> PITGLVYDQRMMLHHNMWDSHHPELPQRISRIFSRHEELRLLSRCHRIPARLATEEELALCHSSKHISIIKSSEHMKPRDLNRLGDEYNSIFISNESYTCALLAAGSCFNSAQAILTGQVRNAVAIVRPPGHHAEKDTACGFCFFNTAALTARYAQSITRESLRVLIVDWDVHHGNGTQHIFEEDDSVLYISLHRYEDGAFFPNSEDANYDKVGLGKGRGYNVNIPWNGGKMGDPEYMAAFHHLVMPIAREFAPELVLVSA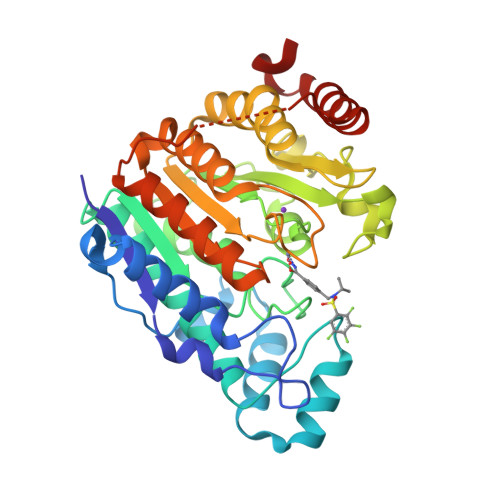GFDAARGDPLGGFQVTPEGYAHLTHQLMSLAAGRVLIILEGGYNLTSISESMSMCTSMLLGDSPPSLDHLTPLKTSATVSINNVLRAHAPFWSSLR>SNRDLFAELSSALVEAKQHSEGKLTLKTHHVNDVGELNISPDEIVSIREQFNMSRGVFARLLHTSSRTLENWEQGRSVPNGQAVTLLKLVQRHPETLSHIAEL[2x];>HMKSVFVESTIFEKY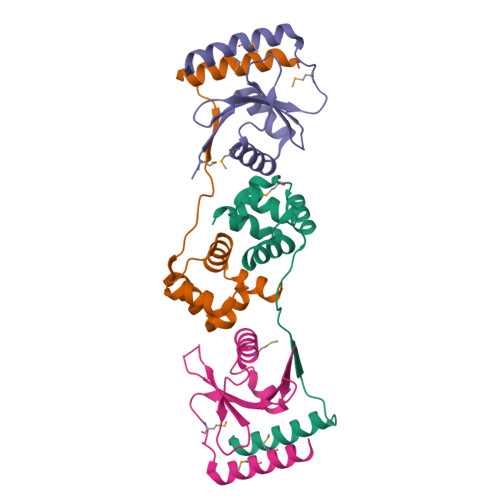RDEYLSDEEYRLFQAELMLNPKLGDVIQGTGGLRKIRVASKGKGKRGGSRIIYYFLDEKRRFYLLTIYGKNEMSDLNANQRKQLMAFMEAWRNEQS[2x]>MSSIGLAHNVTILGSGETTVVLGHGYGTDQSVWKLLVPYLVDDYKVLLYDHMGAGTTNPDYFDFDRYSSLEGYSYDLIAILEEFQVSKCIYVGHSMSSMAAAVASIFRPDLFHKLVMISPTPRLINTEEYYGGFEQKVMDETLRSLDENFKSLSLGTAPLLLACDLESAAMQEYCRTLFNMRPDIACCITRMICGLDLRPYLGHVTVPCHIIQSSNDIMVPVAVGEYLRKNLGGPSVVE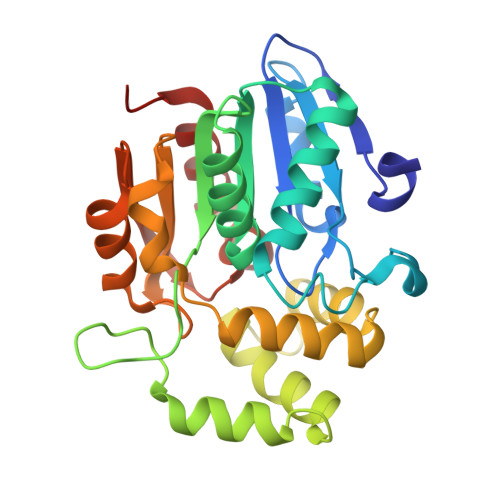VMPTEGHLPHLSMPEVTIPVVLRHIRQDITDH[2x]GUANINE ARABINOSE-5'-PHOSPHATE | C10 H14 N5 O8 P | 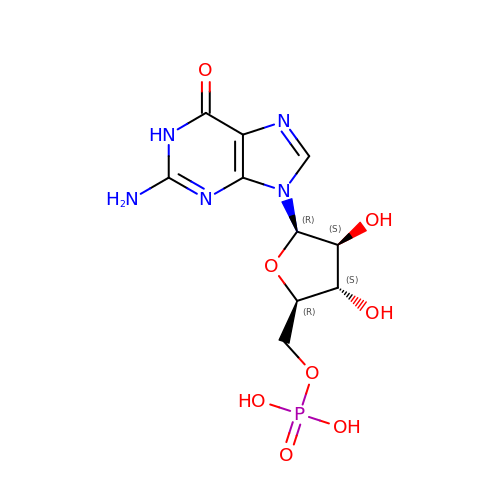RQFCJASXJCIDSX-FJFJXFQQSA-N We have obtained crystals of a racemic compound consisting of l- and d-RNA duplexes in which the enantiomers pack in the crystal lattice in an asymmetric manner and show differences in their structures, crystal contacts and interactions with the solvent. The crystals of d- and l-RNA duplexes (CUGGGCGG)-(CCGCCUGG) belong to space group P1 with the unit cell parameters a = 21.1 Å, b = 26.7 Å, c = 39.1 Å, α = 105.9°, β = 97.0°, and γ = 91.6°. The unit cell contains one d-RNA duplex and one l-RNA duplex stacking head-to-tail, arranged in the crystal lattice into parallel semi-infinite columns. The d-duplexes have the helical parameters characteristic of A-RNA, while the l-duplexes take values appropriately inverted for the other enantiomer.

The absolute configuration of the structure was determined for each analyzed crystal using the anomalous dispersion of X-rays from the Zn2+ ions. Of the nine crystals that gave diffraction data containing statistically significant anomalous signals, seven crystals had the K:L RNA duplex in the d-configuration, and the M:N duplex was in the l-configuration. The remaining two crystals had the inverted configuration l-(K:L)/d-(M:N). Of the eight crystals that gave no statistically significant anomalous signal but gave anomalous peaks at the Zn2+ ions, four crystals were d-(K:L)/l-(M:N), and four were l-(K:L)/d-(M:N). There are no chiral components in the crystallization solution and even if one suspected an unknown contaminant, it should be noted that the crystallization can go ‘either way’, giving crystals of opposite handedness under similar conditions. The two forms are symmetric to each other but asymmetric each in itself. The ratio of the d-(K:L)/l-(M:N) to l-(K:L)/d-(M:N) crystal structures, of 7 to 2 for the best data sets and 11 to 6 overall, does not indicate a clear bias. The intermolecular crystal contacts of the two enantiomers are also different. When the two duplexes (K:L and M:N) are compared, chain K is more exposed to the solvent than its corresponding enantiomer, chain M, which makes more extensive contacts with neighboring RNA molecules. In the presented structure, one enantiomer interacts with three zinc cations, while the other interacts with four zinc cations.

>CUGGGCGG[2x];>[2x]CCGCCUGG>[2x]C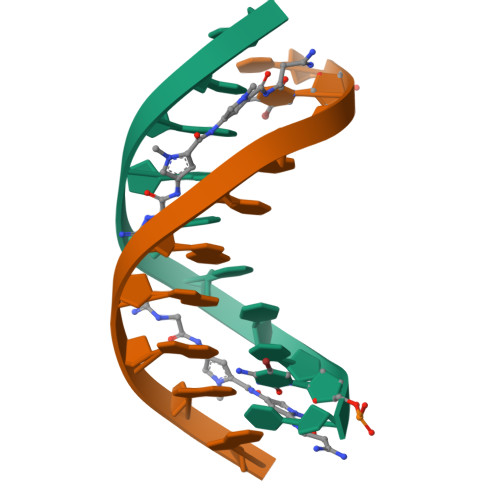CCCCIIIII> GADSPVLMVYGLDQSKMNCDRVFNVFCLYGNVEKVKFMKSKPGAAMVEMADGYAVDRAITHLNNNFMFGQKMNVCVSKQPAIMPGQSYGLEDGSCSYKD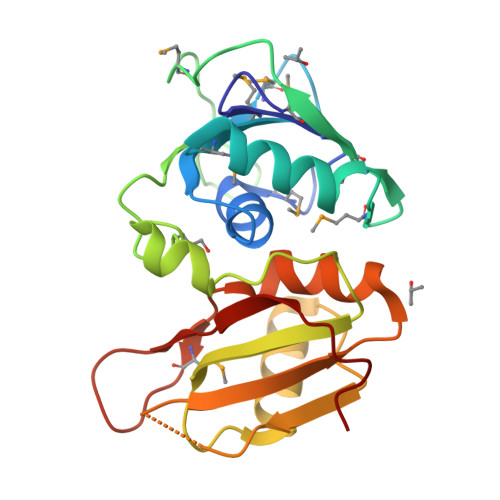FSESRNNRFSTPEQAAKNRIQHPSNVLHFFNAPLEVTEENFFEICDELGVKRPTSVKVFSGKSERSSSGLLEWDSKSDALETLGFLNHYQMKNPNGPYPYTLKLCFSTAQHAS>MDFLRNLFSQTLSLGSQKERLLDELTLEGVARYMQSERCRRVICLVGAGISTSAGIPDFRSPSTGLYDNLEKYHLPYPEAIFEISYFKKHPEPFFALAKELYPGQFKPTICHYFMRLLKDKGLLLRCYTQNIDTLERIAGLEQEDLVEAHGTFYTSHCVSASCRHEYPLSWMKEKIFSEVTPKCEDCQSLVKPDIVFFGESLPARFFSCMQSDFLKVDLLLVMGTSLQVQPFA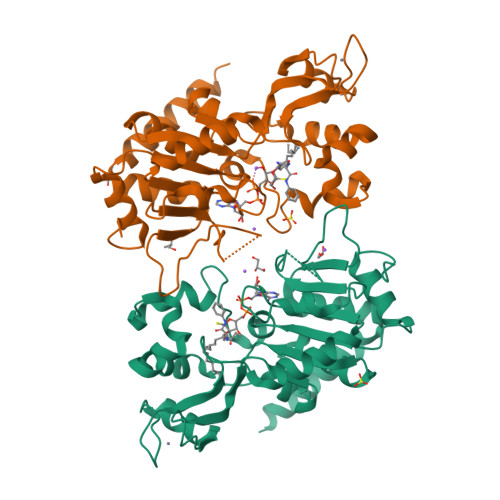SLISKAPLSTPRLLINKEKAGQSDPFLGMIMGLGGGMDFDSKKAYRDVAWLGECDQGCLALAELLGWKKELEDLVRREHASIDAQS[2x]> L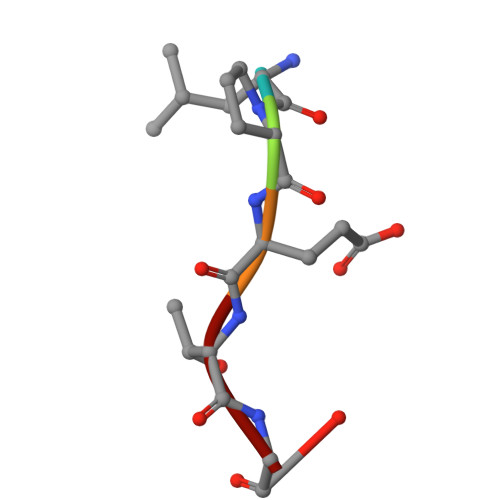PETG>MAHHHHHHMRHQGSSELRSKIMKVAVAGDSAGEGLAKVLADHLKDRFEVSEISRTDAGADAFYANLSD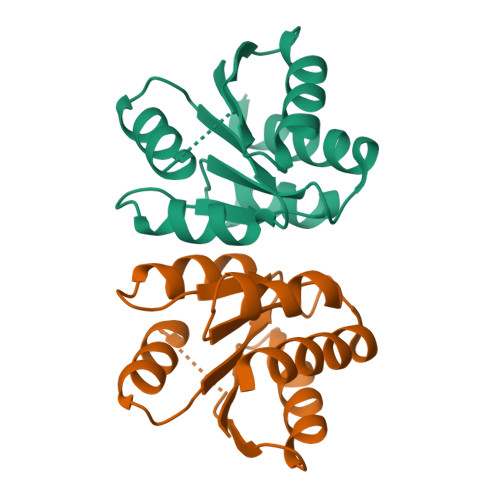RVASAVLDGTYDRAILVCGTGIGVCIAANKVPGIRAALTHDTYSAERAALSNNAQIITMGARVIGAEVAKTIADAFLAQTFDENGRSAGNVNAINEVDAKYNKC[2x]>MSDLKKAAQQAISLMDLTTLNDDDTDQKVIELCHKAKTPAGDTAAICIYPRFIPIARKTLNEIGGDDIKIATVTNFPHGNDDIAIAVLETRAAVAYGADEVDVVFPYRALMEGNETVGFELVKACKEACGEDTILKVIIESGVLADPALIRKASELSIDAGADFIKTSTGKVAVNATLEAAEIMMTVISEKNPKVGFKPAGGVKDAAAAAEFLGVAARLLGDDWATPATFRFGASSLLTNLLHTLELADAPQGAQGYLEHHHHHH[4x]

The 2-deoxy-D-ribose-5-phosphate aldolase (DERA) is an enzyme involved in nucleotide catabolism. The enzyme catalyzes the formation of C-C bonds between an aldehyde as an electrophile and acetaldehyde as a nucleophile in a highly stereoselective manner. The structures display a canonical TIM barrel fold built up of eight β-α repeats in a toroidal arrangement, with an additional N-terminal helix (α0) directly adjacent to the C-terminal helix α8 (vide infra). Furthermore, all DERAs investigated in this study form constitutive dimers.

The X-ray structures of both psychrophilic DERAs were determined with resolutions of 2.1 Å for C. psychrerythraea and 1.8 Å for S. halifaxensis. Superposition of the structures with those of meso- and hyperthermophilic DERAs revealed a high similarity of the monomeric units, with root-mean-square (r.m.s.) deviations (RMSD) in the range of 0.63–1.65 Å. We note that the relative orientations of protomers as well as the characteristics of the dimer interface for both psychrophilic DERAs closely resemble the situation in the mesophilic (E. coli) enzyme. Comparing the substrate binding pockets of the new structures with DERAEC, no amino acid exchanges or significant conformational differences were found within a radius of 5 Å about the natural substrate (as represented by the covalent intermediate included in PDBID 1JCL12). DERAs from psychrophilic species had a similar thermostability and were around 20 K less stable than DERAEC. In contrast, helices 5 and, particularly, 6 and 7 show markedly reduced strengths of rigid contacts in the psychrophilic enzymes. The relative B-factor distribution of the backbone atoms reveals a tendency towards increased flexibility in helices 0, 6, and 7 of the psychrophilic DERAs, compared to DERAEC. Hence, our X-ray structures provide independent clues in favor of the hypothesis that adaption to low temperatures in psychrophilic DERAs involves a more flexible environment of the substrate binding pocket. In the reduced state (i.e., without formation of the disulfide bridge), the A95C mutation turned out to negatively affect the stability of DERASH and DERAEC, but did not influence the stability of DERACP. While in DERASH and DERAEC the melting point of the oxidized form was still lower than the wt value, the exchange led to a marked increase of 8.4 K in thermostability in the case of DERACP.> MRNKIFISHATPDDNDFTRWLALKLIGLGYEVWCDILFLDKGVDFWSNIEKVIREDTCKFLLVSSSYSNQREGVLKELAVAAKVKKQLKDDKFIIPLAIDEQLSYDDINIDIVRLNAIDFKMSWARGLKDILEAFEKQKVPKEVADASKSNLLYQQIFLHDKSVIEKEEIYDSNWLSILSFPEELRFHEYNWMLPKRFDVRELTFPAVRYKNYLCTFAWAYDFTYHLPKTETYHKSKTIRIPTEEILSGSYDSNFIRNAECKRLIVQLLNKAFELRMKDKEVQEYEMSNKTAYWLEKGKLEKDKFEKTMLVGKQKDKNWHFAISGASKLYPFPVLMISSHIFFTADGKKLIDSSSVQHSSRRRQGKNWWNNTWRTKLLAFIKYLSDDDTSFYLEMGSEEKVFVSNEPVKFKGNVSYNIPEKNTLEEEAELSGFNQGEDIEELEELIENLEAE;> MKELIYIEEPKILFAHGQKCTDARDGLALFGPLNNLYGIKSGVIGTKQGLKIFRDYLDHIQKPIYNSNSITRPMFPGFEAVFDCKWESTGITFKEVTNEDIGKFLYNSSTHKRTYDLVSLFIDKIISA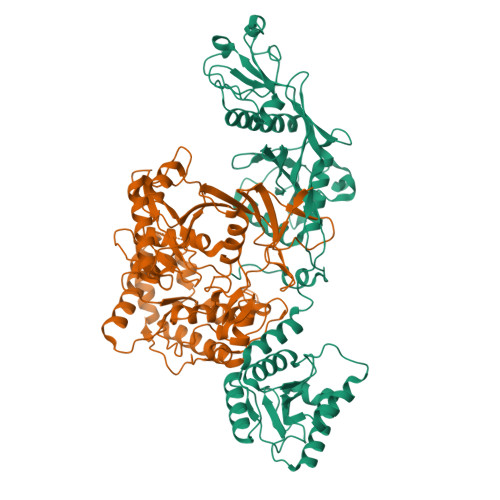NKNEDENVDVWFVIVPDEIYKYCRPNSVLPKEMVQTKALMSKSKAKSFRYEPSLFPDINIELKEQEKEAETYNYDAQFHDQFKARLLKHTIPTQIFRESTLAWRDFKNAFGLPIRDFSKIEGHLAWTISTAAFYKAGGKPWKLSDVRNGVCYLGLVYKKVEKSKNPRNACCAAQMFLDNGDGTVFKGEVGPWYNPKNGQYHLEPKEAKALLSQSLQSYKEQIGEYPKEVFIHAKTRFNHQEWDAFLEVTPKETNLVGVTISKTKPLKLYKTEGDYTILRGNAYVVNERSAFLWTVGYVPKIQTALSMEVPNPLFIEINKGEADIKQVLKDILSLTKLNYNACIFADGEPVTLRFADKIGEILTASTDIKTPPLAFKYYI(2S)-2,4-dihydroxy-N-(3-hydroxypropyl)-3,3-dimethylbutanamide | C9 H19 N O4 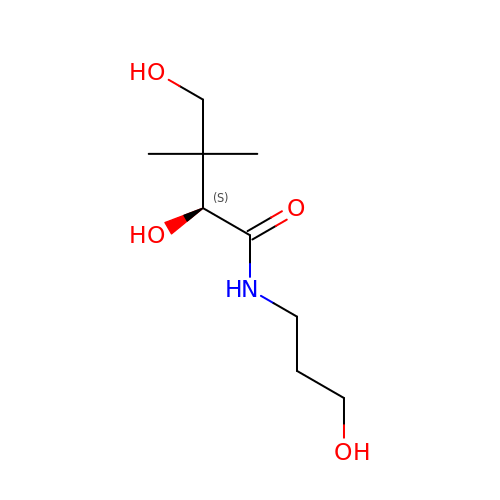| SNPLKNRPJHDVJA-SSDOTTSWSA-N> MEMTSAFTLNVRLDNIAVITIDVPGEKMNTLKAEFASQVRAIIKQLRENKELRGVVFVSAKPDNFIAGADINMIGNCKTAQEAEALARQGQQLMAEIHALPIQVIAAIHGACLGGGLELALACHGRVCTDDPKTVLGLPEVQLGLLPGSGGTQRLPRLIGVSTALEMILTGKQLRAKQALKLGLVDDVVPHSILLEAAVELAKKERPSSRPLPVRERILAGPLGRALLFKMVGKKTEHKTQGNYPATERILEVVETGLAQGTSSGYDAEARAFGELAMTPQSQALRSIFFASTDVKKDPGSDAPPAPLNSVGILGGGLMGGGIAYVTACKAGIPVRIKDINPQGINHALKYSWDQLEGKVRRRHLKASERDKQLALISGTTDYRGFAHRDLIIEAVFENLELKQQMVAEVEQNCAAHTIFASN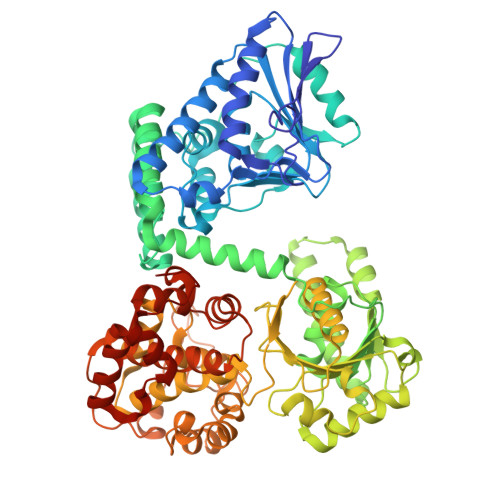TSSLPIGDIAAHATRPEQVIGLHFFSPVEKMPLVEIIPHAGTSAQTIATTVKLAKKQGKTPIVVRDKAGFYVNRILAPYINEAIRMLTQGERVEHIDAALVKFGFPVGPIQLLDEVGIDTGTKIIPVLEAAYGERFSAPANVVSSILNDDRKGRKNGRGFYLYGQKGRKSKKQVDPAIYPLIGTQGQGRISAPQVAERCVMLMLNEAVRCVDEQVIRSVRDGDIGAVFGIGFPPFLGGPFRYIDSLGAGEVVAIMQRLATQYGSRFTPCERLVEMGARGESFWKTTATDLQ>[2x]MGREKTLCKSWSDMKKHLNDTVSKSFIGRFFKLEARKTTFTTELRAATATFLTMAYIITVNANILADSGATCSINDCSTVASSSPPGPECVLGSNPGYEQCISRVKKDLVVATSLSAMVGSLAMGLLANLPFGLAPGMGANAYIAYNVVGFRGSGSISYHTAMAIVLLEGCAFLAVSALGLRGKLARLIPQTVRLACAVGIGMFIAFVGLQMNQGIGLVGPDKSTLVTLTACAETDPVTGACLGGKMKSPTFWLAVVGFLITSFGLMKNVKGSMIYGIVFVTAISWIRGTQVTIFPHTPLGDSNYNYFTKIVDFHKIQSTLGAISFTEFRKSEVWVAFATLFYVDLLGTTGVLYTMAEIGGFVEDGKFEGEYAAYLVDAGS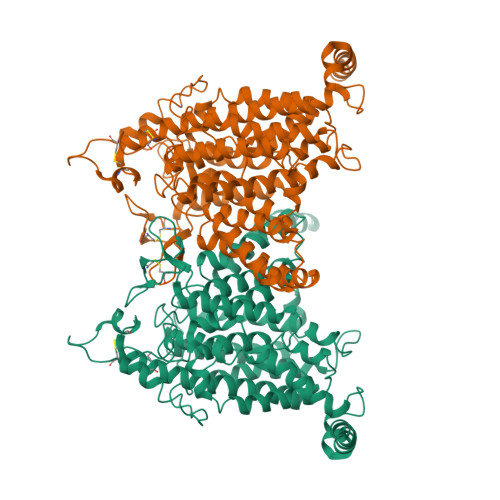SVVGSALGVTTTATFVESSAGLKEGGKTGLTAVIVGLYFLASMFFTPLVTNVPRWAVGPSLVMVGVMMMGVVKDIRWGETKEAVTAFVTILLMPLTYSIANGIIAGIGIYLALSMYDVVLGVAKWLNGVRKRVMREHNQVSSVATVEIV> MMNIVLARIDDRFIHGQILTRWIKVHAADRI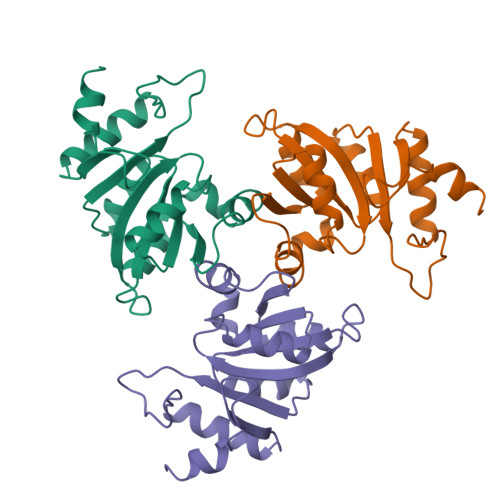IVVSDDIAQDEMRKTLILSVAPSNVKASAVSVSKMAKAFHSPRYEGVTAMLLFENPSDIVSLIEAGVPIKTVNVGGMRFENHRRQITKSVSVTEQDIKAFETLSDKGVKLELRQLPSDASEDFVQILRNVTK> QDLTVKMTDLQTGKPVGTIELSQNDYGVVFIPELADLTPGMHGFHIHQNGSCASSEKDGKVVLGGAAGGHYDPEHTNKHGFPWTDDNHKGDLPALFVSANGLATNPVLAPRLTLKELKGHAIMIHAGGDNHSDMPKALGGGGARVACGV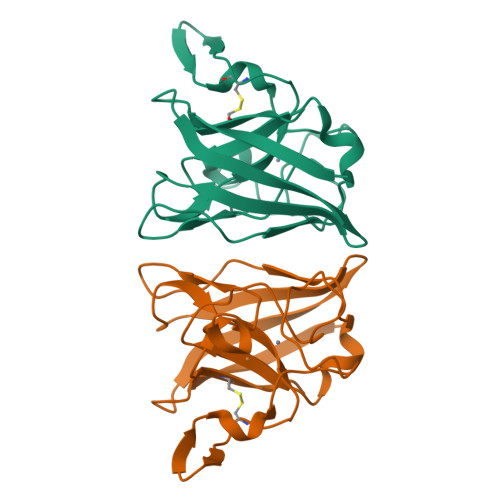IQ The long-wavelength beamline I23 at Diamond Light Source overcomes these limitations and extends the accessible wavelength range to λ = 5.9 Å. In this study, we report the determination of diverse protein structures by experimental phasing techniques carried out at long wavelengths on beamline I23 at Diamond Light Source using S, Ca, K, Cl, V, I, Cd, and P as anomalous scatterers. Native-SAD uses light atoms naturally occurring in proteins or bound to proteins. We demonstrate that long-wavelength native-SAD has become a very compelling technique, where a low multiplicity dataset from a single crystal can be sufficient for successful structure determination, making it a general vehicle of choice for experimental phasing.

Using this protocol, we selected 10 projects solved by S-SAD phasing at the beamline, including soluble and membrane proteins. Structures varied in size with molecular weights ranging from 14 to 114 kDa, sulfur contents varied between 0.9 and 6.5%, and diffraction resolution from 1.8 (detector limited) to 3.4 Å. The overall multiplicity for these datasets was below 26, which is four times lower than the multiplicity typically needed for S-SAD at shorter wavelengths (100)10.

>YSHTATPAITLPSSGSANFAGVEYPLLPLDQHTPLLFQWFERNPSRFGENQIPIINTQQNPYLNNIINAAIIEKERTIGVLVDGNFSAGQKKALAKLEKQYENIKVIYNSDLDYSMYDKKLSDIYLENIAKIEAQPANVRDEYLLGEIKKSLNEVLKNNPEESLVSSHDKRLGHVRFDFYRNLFLLKGSNAFLEAGKHGCHHLQPGGGCIYLDADMLLTGKLGTLYLPDGIAVHVSRKGNSMSLENGIIAVNRSEHPALKKGLEIMHSKPYGDPYIDGVCGGLRHYFNCSIRHNYEEFCNFIEFKHEHIFMDTSSLTISS[4x]>[3x]ASMKDIYVEFRGKYKVDGESRDSEHKGWLEVNSWSHNIRQPKSATSSSVGGHTAERVEHSDMVFVKDLDATSPKLWEACSAGYTFDEVQIDFYRANGDKRIKYLQIKLKHVLVSSVTPTVNEEGVPTEAFGLKYAAVEWTYNQQDINGTAKGAVTKKWSLSNNTASYAALA

Hcp (haemolysin conjugated protein) and VgrG (valine-glycine repeat protein G), products of the genes tssD and tssI, are the homologues of the bacteriophage tail gp19 and the tail spike complex (gp27)3-(gp5)3, respectively. Based in this analogy, these proteins are thought to be molecular markers of a functional T6SS and they may form the needle of this secretion system. Significantly, all of them are composed by a β-barrel forming hexameric rings oligomers with a diameter that can accommodate small folded (< 20 kDa) or unfolded proteins. As described in 2013, many species within the Acinetobacter genus (including non-pathogenic ones) have a conserved and functional T6SS that contains homologues of 12 core T6SS genes, including the hallmarks tssD (Hcp), tssH (ClpV) and tssM.

We also present the structure of Hcp from A. baumannii AB0057 at 1.55 Å resolution, characterizing its self-interactions and oligorimezation. Conversely, the C-terminal tagged Hcp crystals diffracted up to 1.55 Å, the highest resolution as yet reported for a molecule of this type. The Hcp structure revealed a tight β-barrel domain (12 Å diameter) formed by two β-sheets that are comprised of 4 and 5 strands each. The barrel is flanked by a 10-residue α-helix (from Ser70 to Gly80) and a loop, formed by the residues His34 to Asp59, that protrudes more than 25 Å from the core. There are three molecules (0.1 Å RMSD between their Cα atoms) in the asymmetric unit that are packed in a down-up-up fashion, with a distance of 30 Å between chains A and B (head to head arrangement), 20 Å between chains B and C (head to tail) and less than 10 Å between chains C and a symmetry related chain A from the next unit cell (tail to tail). Using the 6-fold crystallographic symmetry, one hexameric ring can be generated from each Hcp chain interacting between them in both, head-to-head and head-to tail behavior. The average contact area between intra-ring molecules is 1325 Å2, with 19 inter-chain hydrogen bonds. The inner diameter of this donut-shaped hexamer is 40 Å and the outer one is 80 Å. Although the A. baumannii Hcp protein forms a nanotube, its packing is unique among these structures, as the 3 chains interact both head-to-tail and head-to-head within the same crystal. All these data suggest that the predominant oligomeric state of Hcp in solution is as a hexamer and hence the model of inter-ring interactions for this structure would be the result of the crystal packing in this particular condition.> MATGTWNEKERKEIPGFYNRFKTQAEKSTNTGLKGRLAMPIRANWGDVGKVV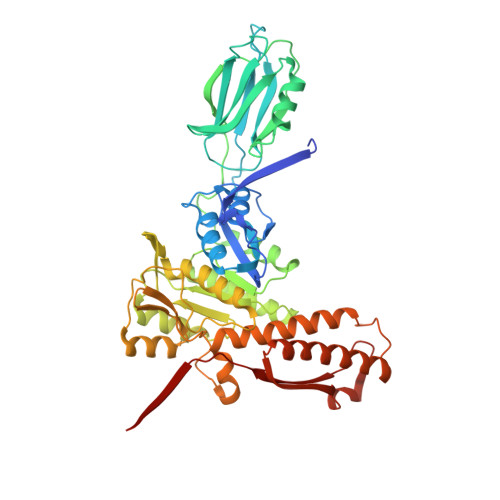TIKNDLRQLKNLFGDDMNYSAFKLGKLALLGNVKELLLYRLVDGNQKKGTLTLKDTTENSAKDVIKLETKYPTARNFNVTIKSNLVDSDKKDFIFFENTKQLFSSSIKGTIDEIVLEINSNLDNEYVIATKVADSDTILANVVNQALEGGNDGCTSITNESYLKALEEFERYSFDSFVLDGVADEALQETTKAWVAKNKELGKDILLFLGGKTEDNIKQINDKSKSFNDENIVNVGSSAYYENIKYTPSEVAVYIAALSVSKGITGSICNAKTIFEEVEPRLSQSEVKECLKSGTLVLDFDDGDVIIVDDVNTFKKYVDDKNEAMGYISNIMFINTINKDTSLKRKEFVGKIFNDATGQTTVICALKKYFEELMSQGIISEFNVDIDTELQATAKADEFYWKWDAVKVDVMKKIYGTGYLG>MAMRRANDPQRREKIIQATLEAVKLYGIHAVTHRKIATLAGVPLGSMTYYFSGIDELLLEAFSSFTEIMSRQYQAFFSDVSDAPGACQAITDMIYSSQVATPDNMELMYQLYALASRKPLLKTVMQNWMQRSQQTLEQWFEPGTARALDAFIEGMTLHFVTDRKPLSREEILRM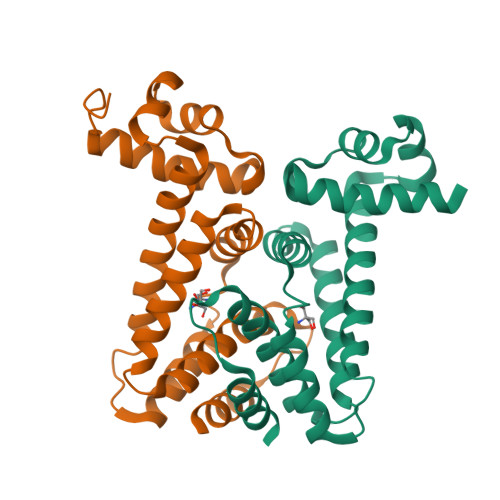VERVAG[2x]> GSADAEYDVVVLGGGPGGYSAAFAAADEGLKVAIVERYKTLGGVCLNVGCIPSKALLHNAAVIDEVRHLAANGIKYPEPELDIDMLRAYKDGVVSRLTGGLAGMAKSRKVDVIQGDGQFLDPHHLEVSLTAGDAYEQAAPTGEKKIVAFKNCIIAAGSRVTKLPFIPEDPRIIDSSGALALKEVPGKLLIIGGGIIGLEMGTVYSTLGSRLDVVEMMDGLMQGADRDLVKVWQKQNEYRFDNIMVNTKTVAVEPKEDGVYVTFEGANAPKEPQRYDAVLVAAGRAPNGKLISAEKAGVAVTDRGFIEVDKQMRTNVPHIYAIGDIVGQPMLAHKAVHEGHVAAENCAGHKAYFDARVIPGVAYTSPEVAWVGETELSAKASARKITKANFPWAASGRAIANGCDKPFTKLIFDAETGRIIGGGIVGPNGGDMIGEVYLAIEMGCDAADIGKTIHPHPTLGESI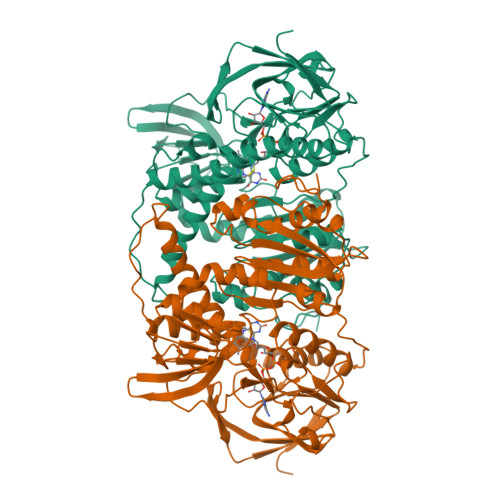GMAAEVALGTCTDLPPQKK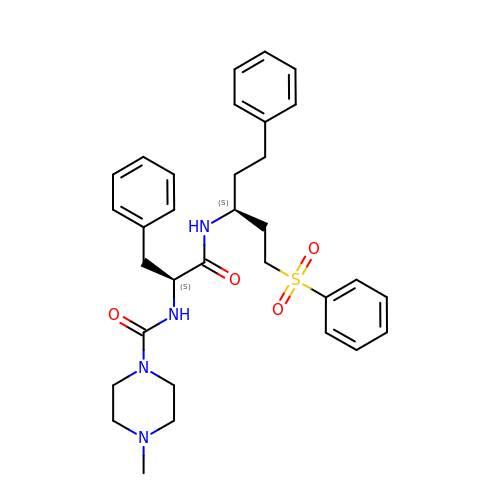Nalpha-[(4-methylpiperazin-1-yl)carbonyl]-N-[(3S)-1-phenyl-5-(phenylsulfonyl)pentan-3-yl]-L-phenylalaninamide | C32 H40 N4 O4 S | VZSXPUDQSLKVIR-JDXGNMNLSA-N>[2x]RELGSNMVHPNVICDGC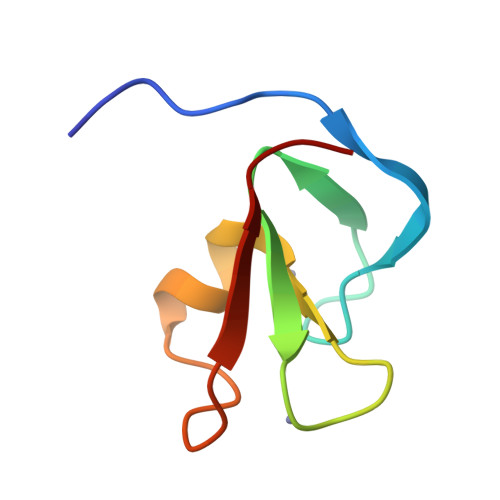NGPVVGTRYKCSVCPDYDLCSVCEGKGLHRGHTKLAFPSP> IVGGYTCGANTVPYQVSLNSGYHFCGGSLINSQWVVSAAHCYKSGIQVRLGEDNI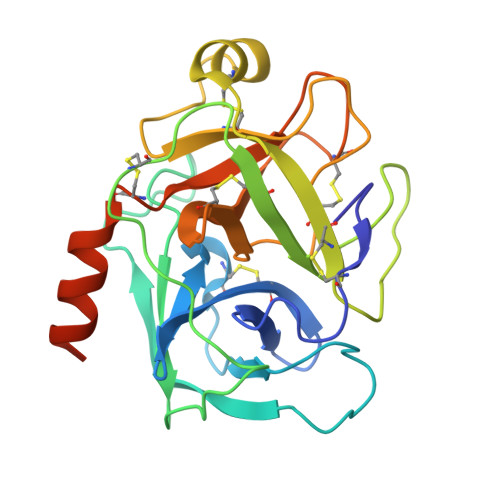NVVEGNEQFISASKSIVHPSYNSNTLNNDIMLIKLKSAASLNSRVASISLPTSCASAGTQCLISGWGNTKSSGTSYPDVLKCLKAPILSDSSCKSAYPGQITSNMFCAGYLEGGKDSCQGDSGGPVVCSGKLQGIVSWGSGCAQKNKPGVYTKVCNYVSWIKQTIASNCNYVSWIKQTIASN>VLPENMKRYMGRDAQRMNILAGRIIAETVRSTLGPKGMDKMLVDDLGDVVVTNDGVTILREMSVEHPAAKMLIEVAKTQEKEVGDGTTTAVVVAGELLRKAEELLDQNVHPTIVVKGYQAAAQKAQELLKTIACEVGAQDKEILTKIAMTSITGKGAEKAKEKLAEIIVEAVSAVVDDEGKVDKDLIKIEKKSGASIDDTELIKGVLVDKERVSAQMPKKVTDAKIALLNCAIEETASEMLKDMVAEIKASGANVLFCQKGIDDLAQHYLAKEGIVAARRVKKSDMEKLAKATGANVIAAIAALSAQDLGDAGLVEERKISGDSMIFVEECKHPKAVTMLIRGTTEHVIEEVARAVDDAVGVVGCTIEDGRIVSGGGS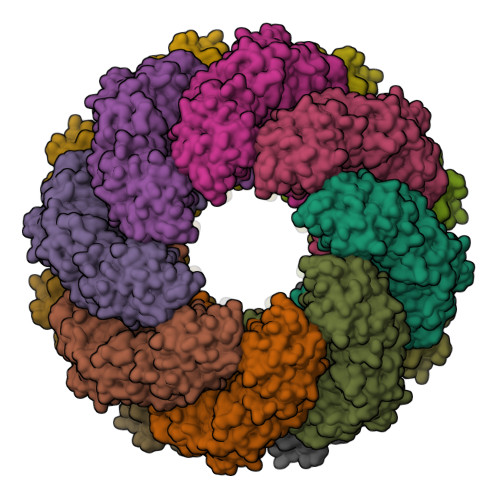TEVELSMKLREYAEGISGREQLAVRAFADALEVIPRTLAENAGLDAIEILVKVRAAHASNGNKCAGLNVFTGAVEDMCENGVVEPLRVKTQAIQSAAESTEMLLRIDDVIAAE[16x]> MSVLEDVFSGKTRIVICGIGNDVRGDDAFGVLVAERLKELVKTPDVLILNCGEMPESYVGKIAAFKPDLVVFVDAIHFGGEIGEFIIADPLKTLGEAVSTHG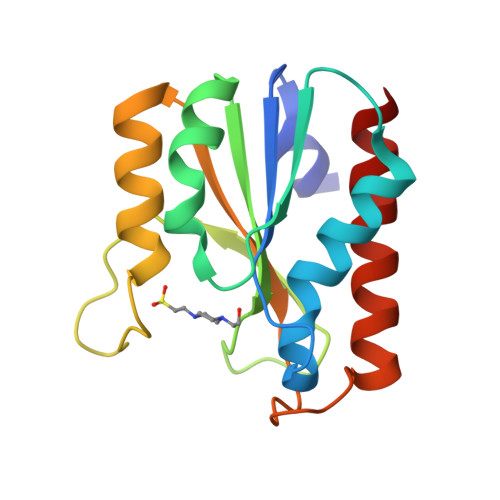LPLRIVASYIKEQTGSDIVLIGCQPGSTGLFEEPSELIKERAERLAELIAEILKNK> MSIATIVPENAVIGQAVNIRSMETDIVSLDDRLLQAFSGSAIATAVDKQTITNRIEDPNLVTDPKELAISQEMISDYNL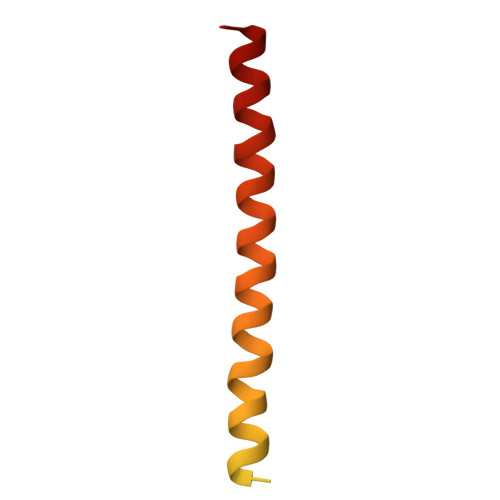YVSMVSTLTRKGVGAVETLLRS> AVYTSEPDVRVPEDKPAKLSCSYSGFSNPRVEWKFAHGDITSLVCYKNKITASYADRVTFSHSGITFHSVTRKDTGTYTCMVSDDGGNTYGEVSVQLTVLVPPSKPTVHIPSSATIGSRAVLTCSEKDGSPPSEYYWFKDGVRMPLEPKGNRAFSNSSYSLNEKTGELVFDPVSAWDTGEYTCEAQ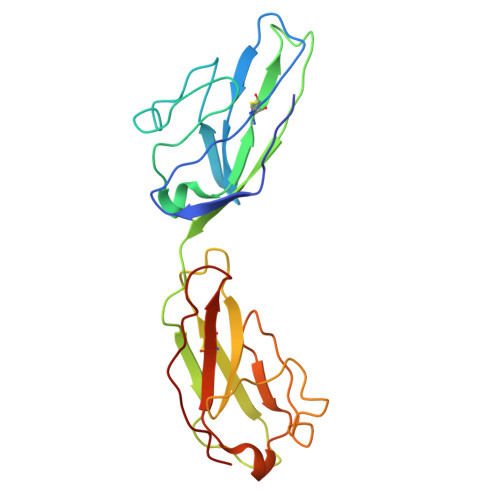NGYGMPMRSEAVRMEA>[4x]MRGSHHHHHTTGEDDESECVINYVEKAVNKLTLQMPYQLFIGGEFVDAEGSKTYNTINPTDGSVICQVSLAQVSDV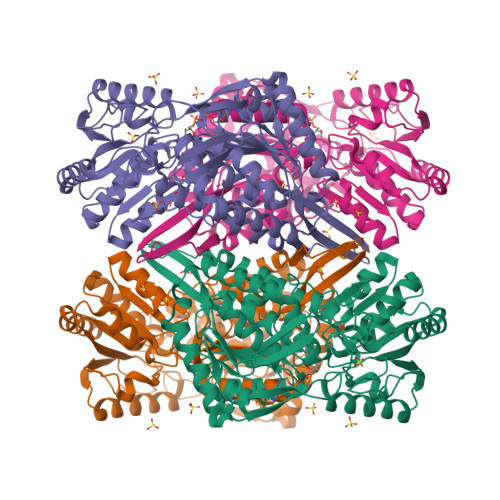DKAVAAAKEAFENGLWGKINARDRGRLLYRLADVMEQHQEELATIEALDAGAVYTLALKTHVGMSIQTFRYFAGWCDKIQGATIPINQARPNRNLTLTKKEPVGVCGIVIPWNYPLMMLSWKTAACLAAGNTVVIKPAQVTPLTALKFAELTLKAGIPKGVVNILPGSGSLVGQRLSDHPDVRKIGFTGSTEVGKHIMKSCALSNVKKVSLELGGKSPLIIFADCDLNKAVQMGMSSVFFNKGENSIAAGRLFVEESIHNQFVQKVVEEVEKMKIGNPLERDTNHGPQNHEAHLRKLVEYCQRGVKEGATLVCGGNQVPRPGFFFQPTVFTDVEDHMYIAKEESFGPIMIISRFADGDVDAVLSRANATEFGLASGVFTRDINKALYVSDKLQAGTVFINTYNKTDVAAPFGGFKQSGFGKDLGEAALNEYLRIKTVTFEY> GSMASQDVIKNLSMNFAKPLEDCKKEMDLPDSVTTDFYNFWKEGYEFTNRQTGCAILCLSSKLELLDQELKLHHGKAQEFAKKHGADDAMAKQLVDLIHGCAQSTPDVADDPCMKT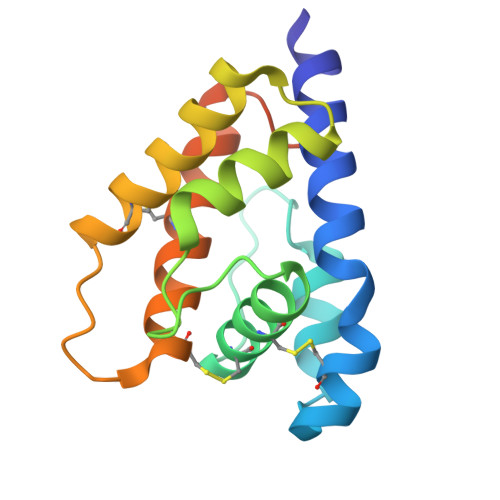LNVAKCFKAKIHELNWAPSMELVVGEVLAEV>[2x]SNAMAKNDKI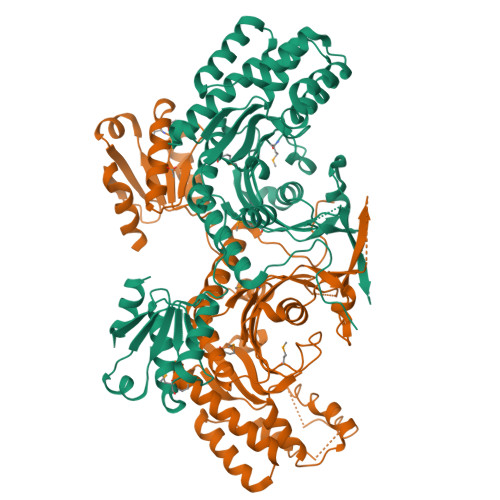NFSTPSGFPEFLPSEKRLELYLLDTIRRVYESYGFTPIETPAVERLEVLQAKGNQGDNIIYGLEPILPPNRQAEKDKSGDTGSEARALKFDQTVPLAAYIARHLNDLTFPFARYQMDVVFRGERAKDGRFRQFRQCDIDVVGREKLSLLYDAQMPAIITEIFEAVNIGDFVIRINNRKVLTGFFQSLNISETQIKSCISIIDNLEKIGEAKVKLELEKEGINPEQTQKIIDFVKIDGSVDDVLDKLKHLSQTLPESEQFNLGVSELETVITGVRNLGVPDKRFCIDLAIARGLNYYTGTVYETTLIGHEALGSICSGGRYEELVGTFIGEKMPGVGISIGLTRLISRLLKAGILNTLPPTPAQVVVVNMQDELMPTYLKVSQQLRQAGLNVITNFEKRQLGKQFQAADKQGIRFCVIIGADEAAAQKSSLKDLQSGEQVEVALADLAEEIKRRLT> TGRPEWIWLALGTALMGLGTLYFLVKGMGVSDPDAKKFYAITTLVPAIAFTMYLSMLLGYGLTMVPFGGEQNPIYWARYADWLFTTPLLLLDLALLVDADQGTILALVGADGIMIGTGLVGALTKVYSYRFVWWAISTAAM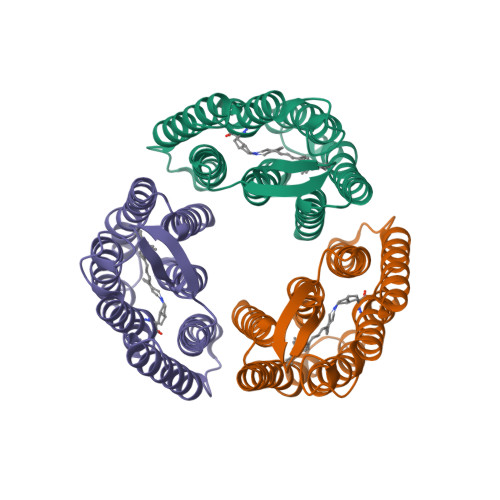LYILYVLFFGFTSKAESMRPEVASTFKVLRNVTVVLWSAYPVVWLIGSEGAGIVPLNIETLLFMVLDVSAKVGFGLILLRSR>[3x]MGQAGEITKYVNPFIGTGAIDGGLSGNNYPGATSPFGMIQLSPDTSEAPNWGDASGYDYNRNTIFGFSHTRLSGTGASDLIDITLMPTSSGRTSSAFTHDEEKARPGYYQVMLKDENINAELTTTQRNGIHRYQYPAGKDAEIILDMDHSADKGSWGRRIINSQIRILNDHAVEGYRIITGWAKLRKIYFYMEFSSPILTSTLRDGGRVHENTAVINGTNLHGCFRFGQLNGKPLTCKVALSSVSMENARQNMEQEAPHWDFDRYVAAADADWEKQLGKIEVKGTEVQKEIFYTALYHTMIQPNTMSDVNGEYMAADYTTRKVANNETHYTTFSLWDTFRASHPLYTLLEPERVTDFVKSMIRQYEYYGYLPIWQLWGQDNYCMIGNHSIPVITDAILKGIPGIDMEKAYEAVYNSSVTSHPNSPFEVWEKYGFMPENIQTQSVSITLEQAFDDWCVAQLAAK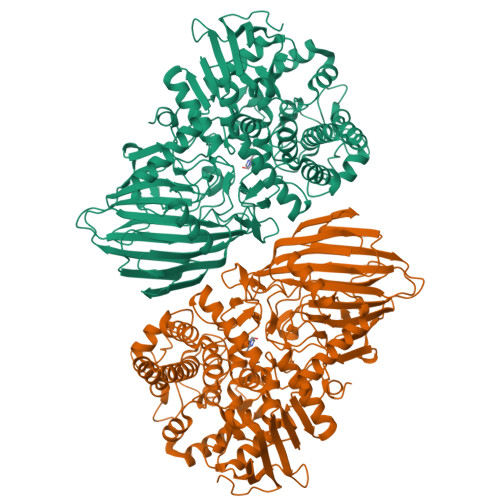LNKDADYQRFHKRSEYYRNLFHPKTKFFQSKNDKGEWIEPFDPYQYGGNGGHPFTEGNAWQYFWYVPHNIQALMELTGGTKAFEQKLDTFFTSTYKSEQMNHNASGFVGQYAHGNEPSHHVAYLYNFAGQPWKTQKYVSHILNTLYNNTSSGYAGNDDCGQMSAWYVFSAMGFYPVNPADGRYIIGSPLLDECTLKLAGNKEFRIRTIRKSPEDIYIQSVTLNGKKHKDFFITHQDIMNGGTMVFKMGKKPSGWGKLEHHHHHH> PISPIETVPVKLKPGMDGPKVKQWPLTEEKIKALVEICTEMEKEGKISKIGPENPYNTPVFAIKKKDSTKWRKLVDFRELNKRTQDFWEVQLGIPHPAGLKKKKSVTVLDVGDAYFSVPLDEDFRKYTAFTIPSINNETPGIRYQYNVL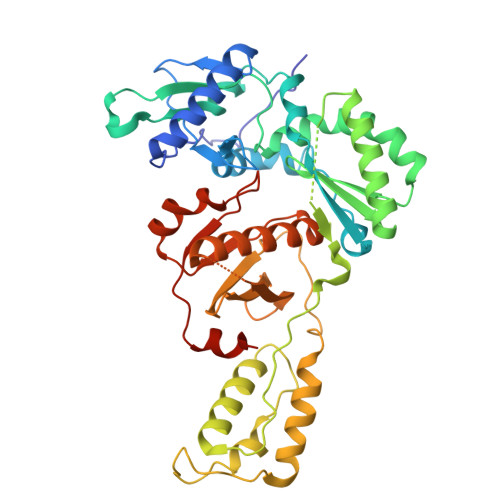PQGWKGSPAIFQSSMTKILEPFRKQNPDIVIYQYMDDLYVGSDLEIGQHRTKIEELRQHLLRWGLTTPDKKHQKEPPFLWMGYELHPDKWTVQPIVLPEKDSWTVNDIQKLVGKLNWASQIYPGIKVRQLCKLLRGTKALTEVIPLTEEAELELAENREILKEPVHGVYYDPSKDLIAEIQKQGQGQWTYQIYQEPFKNLKTGKYARMRGAHTNDVKQLTEAVQKITTESIVIWGKTPKFKLPIQKETWETWWTEYWQATWIPEWEFVNTPPLVKLWYQLEKEPIVGAETF> GSHMTWLSDFPQAWAETGGMGLAVRQAPLIIPLKATSTPVSIKQYPMSQEARLGIKPHIQRLLDQGILVPCQSPWNTPLLPVKKPGTNDYRPVQDLREVNKRVEDIHPTVPNPYNLLSG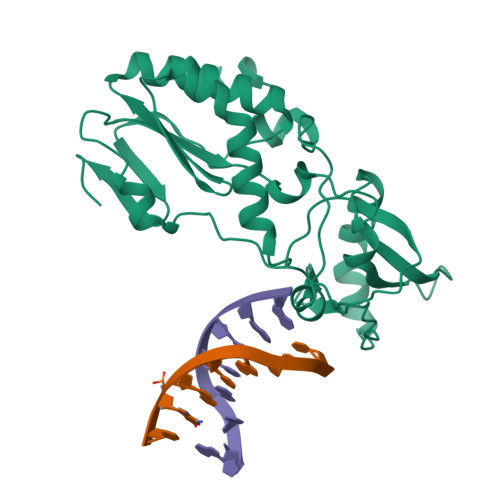LPPSHQWYTVLDLKDAFFCLRLHPTSQPLFAFEWRDPEMGISGQLTWTRLPQGFKNSPTLFDEALHRDLADFRIQHPDLILLQYVDDLLLAATSELDCQQGTRALLQTLGNLGYRASAKKAQICQKQVKYLGYLLKEGQR1,1,1,3,3,3-HEXAFLUOROPROPANEDIOL 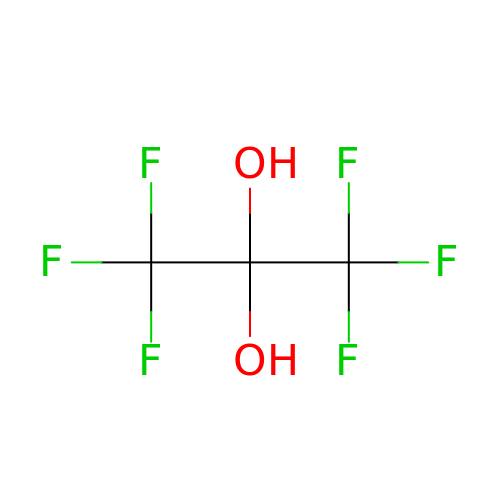| C3 H2 F6 O2 | AKVXSYUWYXOLMY-UHFFFAOYSA-N>[2x]GPNDNLEAELEQTKALCEVAKQLRKLPLLTEERRFEAVGALEESKK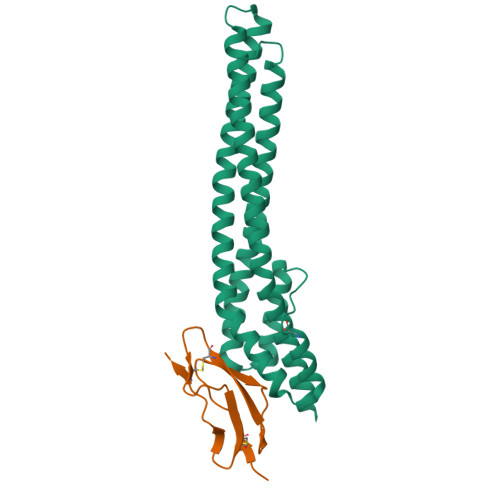AAKEGKKAAKRAEAGAVGGTSEQQQAAKRAREAATVAYEASVRAEAAAMEVKRFARALDSFESEYESVFSGLLRGAAEHGGNETIKQLAKECATAVADDVTPEALTRAAHNLRGLYMQDFAEEYLQEANEAANKLEELQKATAETVRAADAADDAKSEAQEEAAQFPEIDDDDSDEDKEDEAS;>GEITCDPPRIPNGVYRPELSKYRGQDKITYECKKGFFPEIRGTDATCTRDGWVPVPRCAWK[2x]> GPLGSGAGDGAPVGLDLDRLARDCDVVGGQLALHHQGTLTTWEFGTEEHAGGRPVHVGSAFPYGSVTKAFTATAVLQLAGDGDLDLDRPVRELLPEAEAEAEIEVEAGSGTGARADGGHPALAATLRQLLSHTAGLPSDHDDERAPSLRRWLTGFLALPVGPWPAPGSFSYSNVGYGIAGRVVEAVTGLTWSEAVRDFLLHPLGTAITVLPTDPGSLPAGGLAGSAADLVRLGRLHLDEPGDPDLARLADPDALREMARPTAGADPFGLADGWGPGLGRFGPAGNRWLGHDGTLDGATCHLRIHPGRGTVVALTTNSPTGQALWDAVVDALRDADIDVGVHRPAPPPAIAAAAFADCTGTYR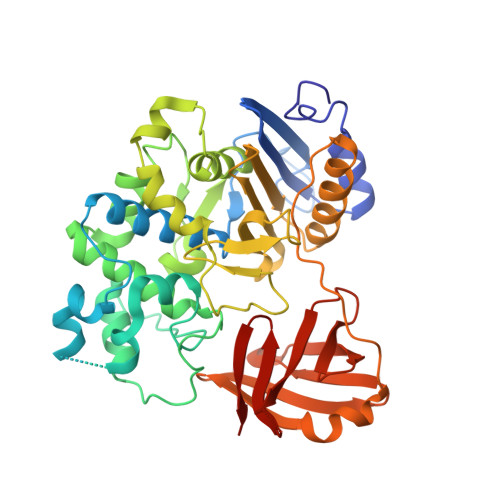NGDLAVTVGIDGPYLVLELPGGARELAQPLAHRTFSSRGAGFLGRFVTDARSDAVHALQYSGRTLLREAGES3-azanyl-2-(phenylmethyl)benzo[f]quinoxalin-8-ol | 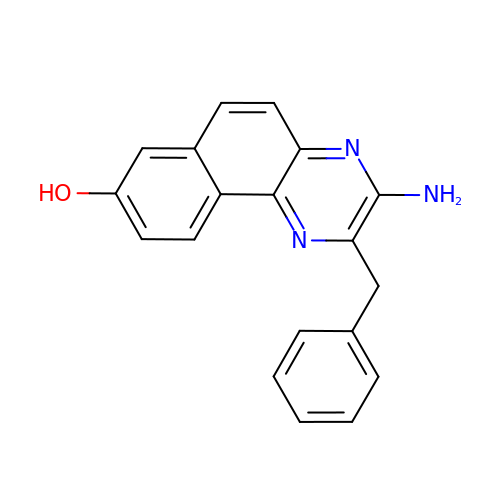C19 H15 N3 O | FZAJVBZJLFLZOR-UHFFFAOYSA-N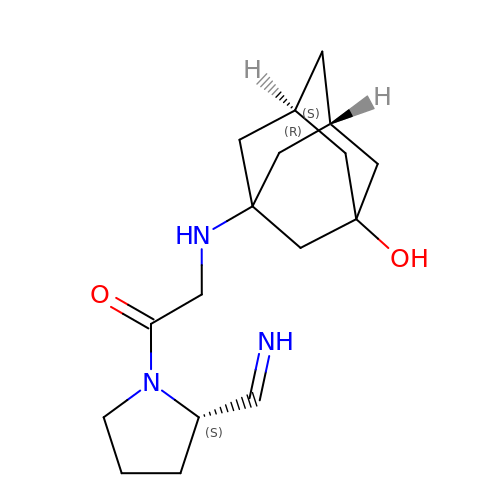2-{[(1r,3s,5R,7S)-3-hydroxytricyclo[3.3.1.1~3,7~]decan-1-yl]amino}-1-{(2S)-2-[(E)-iminomethyl]pyrrolidin-1-yl}ethan-1-one | C17 H27 N3 O2 | LUWVSODOPBYGON-FEZPVXCISA-N Potassium ion (K+) channels are highly selective membrane protein pores and operate with near diffusion limited efficacy. Their high selectivity and flow rates allow them to function as critical elements in electrically excitable cells, such as neurons, muscle cells, and endocrine cells, facilitating the use of electricity in biological organisms. Each subunit contributes a linear backbone consisting of five or six residues with their carbonyl groups pointing inward to generate a fourfold symmetrical binding pore.

The correlation between the atomic displacement parameters (ADPs) and the occupancy of an atom coupled with the inability to distinguish between electron density of a K+ ion and that of a water molecule make anomalous diffraction studies necessary. To fully understand the characteristics of K+ movement in a single file through the channel, we have experimentally determined the number of K+ ions within a selectivity filter, using anomalous X-ray diffraction. Despite the long wavelength of λ = 3.35 Å the data was of high quality allowing the crystallographic phase problem to be solved by K-SAD. Using the SAD data directly, we were able to refine the occupancy of the four K+ ions within the ion channel in each of two protein molecules (subunit A and subunit B) present in the crystallographic asymmetric unit, with the phenix.refine program. Each K+ ion within the selectivity filter is shared between four unit cells and thus has a maximum occupancy value of 0.25. All of the four K+ ions in the channel refine to occupancy values close to the maximum possible value (0.25) with ADPs that are almost identical to the oxygen atoms located at the sides of the ion channel with which they are interacting. Phenix.refine refines occupancies and ADP (or B-factors) separately at all times. After refinement, the occupancy values for all the K+ ions in the channel clustered around 0.25, suggesting that all four K+ binding sites in the NaK2K selectivity filter are fully occupied with K+ ions. The high K+ ion refined occupancies at all sites in the selectivity filter indicate that all sites are fully occupied with K+ ions with a total of four K+ ions being present within the selectivity filter at a K+ ion concentration of 100 mM. These results suggest that water is not co-translocated with K+ ions, which is seemingly in disagreement with ion/water co-translocation ratios determined from earlier experiments. However, it is in total agreement with earlier molecular dynamics simulations and crystallographic data analysis, suggesting that ion transport occurs via direct coulomb knock-on.

>KDKEFQVLFVLTILTLISGTIFYSTVEGLRPIDALYFSVVTLTTVGYGDFSPQTDFGKIFTILYIFIGIGLVFGFIHKLAVNVQLPSILSNLVPR[2x]> MPLRKMKIPFLLLFFLWEAESHAASRPNIILVMADDLGIGDPGCYGNKTIRTPNIDRLASGGVKLTQHLAASPLATPSRAAFMTGRYPVRSGMASWSRTGVFLFTASSGGLPTDEITFAKLLKDQGYSTALIGKWHLGMSCHSKTDFCHHPLHHGFNYFYGISLTNLRDCKPGEGSVFTTGFKRLVFLPLQIVGVTLLTLAALNCLGLLHVPLGVFFSLLFLAALILTLFLGFLHYFRPLNCFMMRNYEIIQQPMSYDNLTQRLTVEAAQFIQRNTETPFLLVLSYLHVHTALFSSKDFAGKSQHGVYGDAVEEMDWSVGQILNLLDELRLANDTLIYFTSDQGAHVEEVSSKGEIHGGSNGIYKGGKANNWEGGIRVPGILRWPRVIQAGQKIDEPTSNMDIFPTVAKLAGAPLPEDRIIDGRDLMPLLEGKSQRSDHEFLFHYCNAYLNAVRWHPQNSTSIW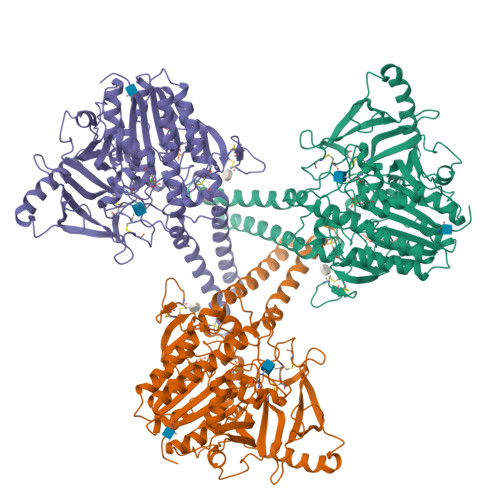KAFFFTPNFNPVGSNGCFATHVCFCFGSYVTHHDPPLLFDISKDPRERNPLTPASEPRFYEILKVMQEAADRHTQTLPEVPDQFSWNNFLWKPWLQLCCPSTGLSCQCDREKQDKRLSR To gain further insight into the structural conversions in pore formation, we chose pleurotolysin (Ply), a MACPF protein consisting of two components, PlyA and PlyB, from Pleurotus ostreatus. Previous studies have shown that PlyA binds membranes and is required to recruit the pore-forming MACPF protein PlyB to the membrane surface. PlyA and PlyB together form relatively small and regular pores in liposomes. The membrane attack complex/perforin-like family (MACPF) proteins form the largest superfamily of pore-forming proteins identified to date.

The 1.85 Å X-ray crystal structure of PlyA revealed a β-sandwich fold, unexpectedly related to the actinoporin-like family of pore-forming toxins. Previous studies suggest that actinoporin-like proteins interact with membranes via one end of the β-sandwich, with the N-terminal sequence responsible for forming the pore. However, PlyA lacks the proposed actinoporin N-terminal transmembrane region consistent with the observation that PlyA binds membranes, but is unable to form pores on its own. However, in the crystal structure of PlyA, we noted two different V-shaped dimers (termed N-dimer and C-dimer) in the asymmetric unit. Both forms fitted adequately into EM density, placing either the PlyA N-terminus (N-dimer) or C-terminus (C-dimer) in proximity to the membrane surface. We tested the orientation of PlyA by adding a hexahistidine tag to the N-terminus, which abrogated membrane binding of PlyA to red blood cells whereas a C-terminal tag had no effect on binding. Also, mutation of Trp 6 (W6E), located in the PlyA N-dimer interface, reduced membrane binding and led to 100-fold lower pore-forming activity (Fig. 4A, denoted as purple spheres).

>[4x]MAYAQWVIIIIHNVGSKDVKIKNLKPSWGKLHADGDKDTEVSASKYEGTVIKPDEKLQINACGRSDAAEGTTGTFDLVDPADGDKQVRHFYWDCPWGSKTNTWTVSGSNTKWMIEYSGQNLDSGALGTITVDTLKKGN(1~{S},2~{S},3~{S},4~{S})-4-(hydroxymethyl)cyclopentane-1,2,3-triol 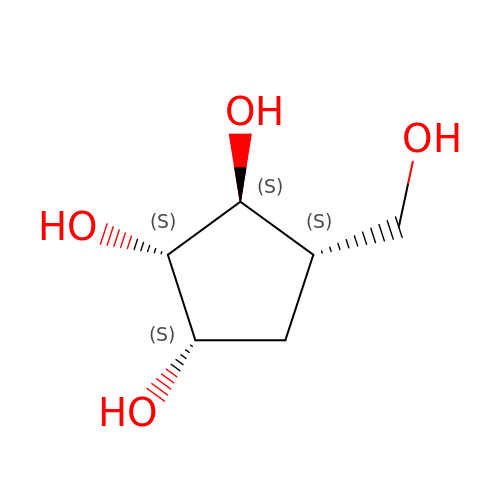| C6 H12 O4 | PHKHGSSZAJVEQK-BXKVDMCESA-N>[2x]MVEKGKMVKISYDGYVDGKLFDTTNEELAKKEGIYNPAMIYGPVAIFAGEGQVLPGLDEAILEMDVGEER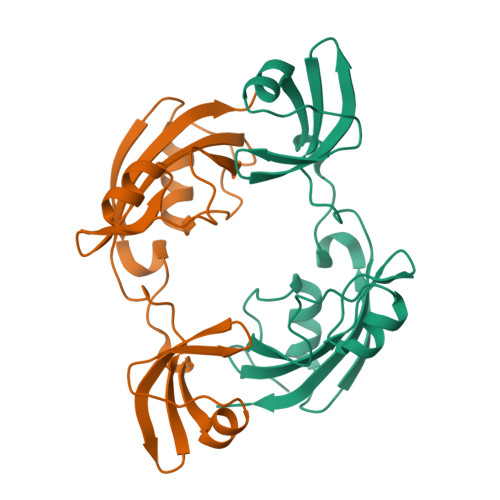EVVLPPEKAFGKRDPSKIKLIPLSEFTKRGIKPIKGLTITIDGIPGKIVSINSGRVLVDFNHELAGKEVKYRIKIEEVVDLHHHHHH> AASGSALIFDEEMSRYKLLWTDPECEIEVPERLTVSYEALRTHGLAQRCKAVPVRQATEQEILLAHSEEYLEAVKQTPGMNVEEL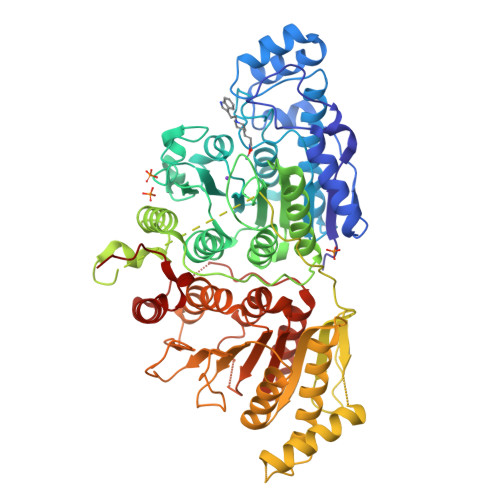MAFSKKYNAVYFHQNIYHCAKLAAGATLQLVDSVMKREVRNGMALVRPPGHHSQRSAANGFCVFNNVAFAALYAKKNYNLNRILIVDWDVHHGQGIQYCFEEDPSVLYFSWHRYEHQSFWPNLPESDYSSVGKGKGSGFNINLPWNKVGMTNSDYLAAFFHVLLPVAYEFDPELVIVSAGFDSAIGDPEGEMCALPEIFAHLTHLLMPLAAGKMCVVLEGGYNLTSLGQSVCQTVHSLLGDPTPRISGLGTACDSALESIQNVRNVQSSYWSSFKHLAQSETNPKRPRLDATNGGPKESSEPASESNPKKTAQDIVWPEPLKRMPASVRTVVVPPPGVELTLPKNCQHSGDISESTAKEVQRIRDKHFHDLTDQNILRSLGNIISVLDRMMRSDEVCNGCVVVSDLSVSVQCALQHALTEPAERVLVVYVGDGELPVKTNDGKVFLVQICTKETEDKCVNRLTLCLREGESLTAGFMQALLGLILPVAYEFNPALVLGIVEETAAKTRLMRVWGHMTCLIQGLARGRMLTLLQGYDKDLLELTVSALSGASISPLGPLRAPKPEDVEMMEKQRQRLQERWGLLRCTVSESW> GASMTIEDEYSGPKLEDGKVTISFMKELMQWYKDQKKLHRKCAYQ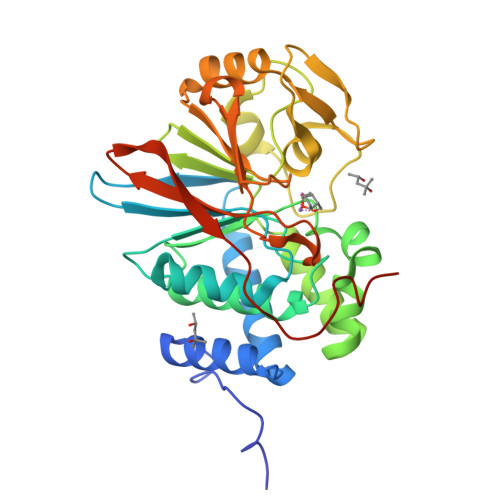ILVQVKEVLSKLSTLVETTLKETEKITVCGDTHGQFYDLLNIFELNGLPSETNPYIFNGDFVDRGSFSVEVILTLFGFKLLYPDHFHLLRGNHETDNMNQIYGFEGEVKAKYTAQMYELFSEVFEWLPLAQCINGKVLIMHGGLFSEDGVTLDDIRKIERNRQPPDSGPMCDLLWSDPQPQNGRSISKRGVSCQFGPDVTKAFLEENNLDYIIRSHEVKAEGYEVAHGGRCVTVFSAPNYCDQMGNKASYIHLQGSDLRPQFHQFTAVPHPNVKPMAYANTLLQLGMM Functionally, as a group I chaperonin in mitochondria, mtHsp60 forms a complex with the cochaperonin mtHsp10 (gene name: HSPE1) and serves as folding machinery by facilitating the proper folding of unfolded proteins. In addition, because mtHsp60-Hsp10 complex is the eukaryotic homolog of bacterial chaperonin, GroEL:ES, it has similar biochemical properties with GroEL:ES directing the substrate folding process using their well conserved hydrophobic residues (10–12). Mitochondrial heat shock protein 60 (mtHsp60; gene name: HSPD1) is one of the proteins whose expression level is notably increased through mtUPR yet it is the most abundant protein under basal condition within mitochondria. Because of its abundance and functional role, the mtHsp60-Hsp10 complex is considered as a crucial factor to mitigate folding stress.

To characterize the detailed in situ structural properties of the mtHsp60-Hsp10 complex under folding stress, we performed subtomogram averaging using particles extracted from stressed mitochondria. We focused primarily on the football conformation, as the half-football and bullet-like conformations were present at low abundance, yielding poorly resolved reconstructions. The structure exhibits the classical features of a football shaped group I double-ring chaperonin: 14 mtHsp60 subunits arranged in two stacked rings of seven each, capped by a heptameric mtHsp10 (10, 11, 28). The in situ structures closely resemble a previously reported in vitro cryo-EM structure of a purified mtHsp60 complex in a similar football-shaped arrangement. Our analysis suggests that, in situ, the ATP-binding sites in the Hsp60-Hsp10 complex are not fully occupied, with ~12 of the 14 nucleotide-binding pockets showing evidence of occupancy, which indicates that fully occupied nucleotide is not necessary for its function and formation of football complex. With the fitted model, we identified the extra density as potential salt bridges between residues Lys103 and Glu107, as well as Arg444 and Glu460. Under folding stress, we also observed structural asymmetry and substrate-dependent contacts involving conserved hydrophobic residues—such as Phe279, Tyr359, and Trp42—lining the inner chamber, indicating active substrate engagement. In addition, we observed extra density at the base of the chamber, primarily located in the region of the unstructured C-terminal tails (residues 523 to 547) of mtHsp60 subunits, which displays connectivity to the substrate density. Notably, folding stress led to a significant increase in the proportion of the football conformation. These results suggest that under folding stress, the mtHsp60-Hsp10 complex increases its proportion of the football conformation as a structural response to elevated levels of unfolded proteins, thereby enhancing its folding capacity.

>[14x]MAGQAFRKFLPLFDRVLVERSAAETVTKGGIMLPEKSQGKVLQATVVAVGSGSKGKGGEIQPVSVKVGDKVLLPEYGGTKVVLDDKDYFLFRDGDILGKYVD;>[14x]MLRLPTVFRQMRPVSRVLAPHLTRAYAKDVKFGADARALMLQGVDLLADAVAVTMGPKGRTVIIEQSWGSPKVTKDGVTVAKSIDLKDKYKNIGAKLVQDVANNTNEEAGDGTTTATVLARSIAKEGFEKISKGANPVEIRRGVMLAVDAVIAELKKQSKPVTTPEEIAQVATISANGDKEIGNIISDAMKKVGRKGVITVKDGKTLNDELEIIEGMKFDRGYISPYFINTSKGQKCEFQDAYVLLSEKKISSIQSIVPALEIANAHRKPLVIIAEDVDGEALSTLVLNRLKVGLQVVAVKAPGFGDNRKNQLKDMAIATGGAVFGEEGLTLNLEDVQPHDLGKVGEVIVTKDDAMLLKGKGDKAQIEKRIQEIIEQLDVTTSEYEKEKLNERLAKLSDGVAVLKVGGTSDVEVNEKKDRVTDALNATRAAVEEGIVLGGGCALLRCIPALDSLTPANEDQKIGIEIIKRTLKIPAMTIAKNAGVEGSLIVEKIMQSSSEVGYDAMAGDFVNMVEKGIIDPTKVVRTALLDAAGVASLLTTAEVVVTEIPKEEKDPGMGAMGGMGGGMGGGMF> EL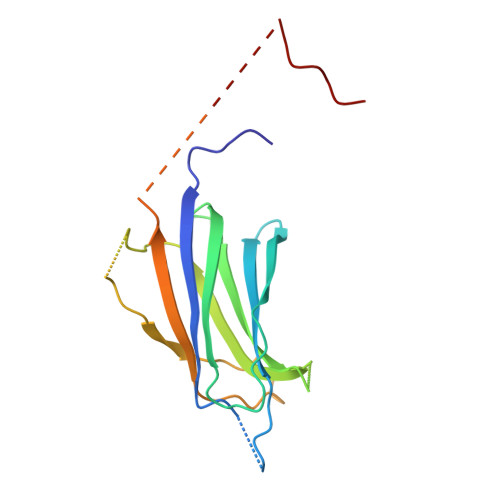HNDDTRVVRVKVIAGIGLAKKDILGASDPYVRVTLYDPMSGILTSVQTKTIKKSLNPKWNEEILFRVLPQRHRILFEVFDENRLTRDDFLGQVDVPLYPLPTENPRMERPYTFKDFVLHPRSHKSRVKGYLRLKMTYLPKNGSEDENADQAEELEPGWVVLDQPDAATHLPHPP1-{5-[2-chloro-5-(hydroxymethyl)phenyl]pyridin-2-yl}piperidine-4-carboxylic 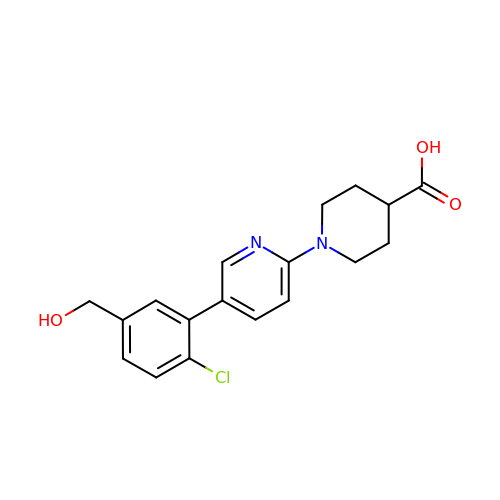acid | C18 H19 Cl N2 O3 | ZHEDDGBFOGXDOY-UHFFFAOYSA-N>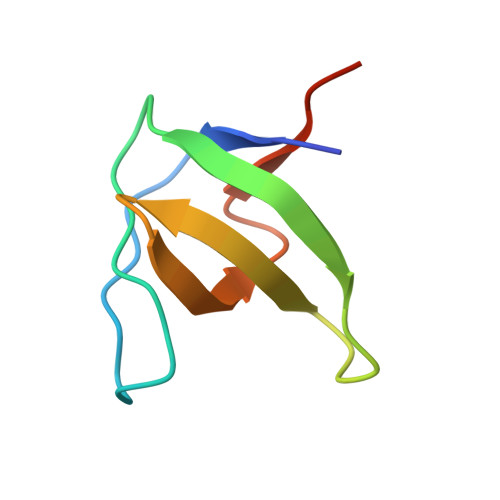 MVDYIVEYDYDAVHDDELTIRVGEIIRNVKKLQEEGWLEGELNGRRGMFPDNFVKEIKRETE> MEQTQKLKLNLQHFASNNVKPQVFNPDNVMMHEKKDGTLMNEFTTPILQEVMENSKIMQLGKYEPMEGTEKKFTFWADKPGAYWVGEGQKIETSKATWVNATMRAFKLGVILPVTKEFLNYTYSQFFEEMKPMIAEAFYKKFDEAGILNQGNNPFGKSIAQSIEKTNKVIKGDFTQDNIIDLEALLEDDELEANAFISKTQNRSLLRKIVDPETKERIYDRNSDSLDGLPVVNLKSSNLKRGELITGDFDKLIYGIPQLIEYKIDETAQLSTVKNEDGTPVNLFEQDMVAL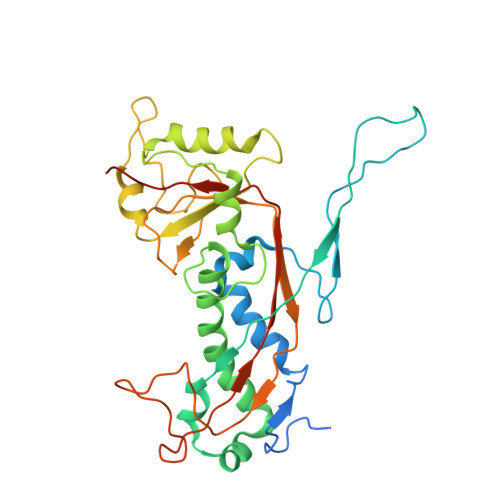RATMHVALHIADDKAFAKLVPADKRTDSVPGEV>[2x]MTIVNRIRTDVVNVAKSFGAEYSEAVIDQIFQGFGEKFTNTGFAIRVQNKRNQKVDCNIRYGEAKENCLAWDIARESGLLSDQGHPVDTLIQEMFQAIPAIAYGADFDINYGLVKIWHLPKIVPVEEAFKIPSLPKSV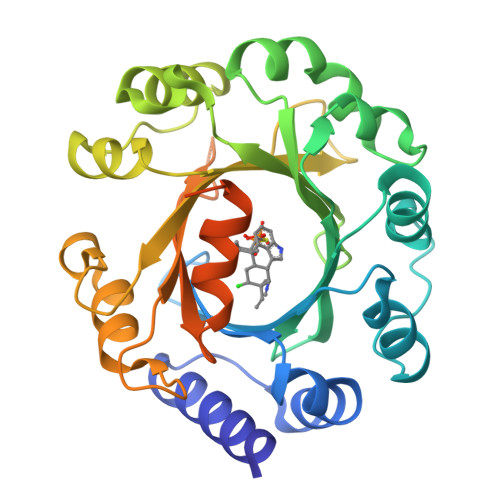NAHIDFFKKYHLDALCALTVDYRNKSTNLYFDAHHPEQRTTQFYKNILQSQQFEVPSDEVLEILVNCPEIAVTFNWSSPGIERMCFYTAFVNRETVPQHINPVLKKFAQEAPALLDNPGFLVGWSFGPDAKKGTYIKIDVDYHGLVVPSFFHMHNLPLPIPEANSVFDLPSSDTEDKLNSIVMSKLAAALEHHHHHH> KPEPTDEEWELIKTVTEAHVATNAQGSHWKQKRKFLPEDIGQAPIVNAPEGGKVDLEAFSHFTKIITPAITRVVDFAKKLPMFCELPCEDQIILLKGCCMEIMSLRAAVRYDPESETLTLNGEMAVTRGQLKNGGLGVVSDAIFDLGMSLSSFNLDDTEVALLQAVLLMSSDRPGLACVERIEKYQDSFLLAFEHYINYRKHHVTHFWPKLLMKVTDLRMIGACLASRFLHMKVECPTELFPPLFLEVF;> ENALLRYLLDK

The thyroid hormone receptors (THRs) are nuclear hormone receptors regulated by endogenous thyroid hormones, including the inactive prohormone thyroxine (T4) and the bioactive hormone 3,3′,5-triiodothyronine (T3), which are critical for development regulation and metabolic homeostasis. As ligand-regulated nuclear receptors, THRs have a structurally conserved LBD that allows the binding of distinct ligands (Burris et al., 2013). Following the ligand binding, the function of THRs is mediated through the selective recruitment or release of specific coregulators, like the family of steroid receptor coactivators (SRCs) (Li et al., 2003, Jin and Li, 2010, Savkur and Burris, 2004), as a heterodimeric complex with retinoid X receptor (RXR) (Putcha et al., 2012, Kojetin et al., 2015, Mangelsdorf and Evans, 1995). Although the defects in any of the processes in thyroid hormone transport and synthesis can all contribute to RTH, in most cases the disorder involves defective thyroid hormone receptors, resulting in reduced T3 binding and disruptive thyroid hormone signaling.

As expected, the native ligand T3 abolished or substantially diminished the transcriptional activity of four THRβ mutants associated with thyroid hormone resistance, V264D, H435L, R438H, and R438W, respectively (Wakasaki et al., 2016, Nomura et al., 1996, Sabet and Pallotta, 2011, Narumi et al., 2010). Surprisingly, the treatment of roxadustat either enhanced or retained the transcriptional activity of these THRβ mutants, all leading to higher induced transcriptional activity than those of T3. In contrast, the binding of roxadustat resulted in higher Tm values for four TRβ mutants than that of T3. Although all four mutant residues are located in the THRβ LBD, H435 is the only one that directly contacts ligands T3 or roxadustat, whereas the rest of the mutant residues are located outside the ligand-binding pocket, not in the range to form intimate contacts with the ligands, which makes us wonder how these mutants influence the ligand binding. To unravel the molecular basis for the RTH of the THRβ mutants and further their beneficial susceptibility to roxadustat, we performed structural studies on the THRβ mutants complexed with roxadustat. The structural analysis further revealed an apparent conformational change of residue H435 on helix 10 of THRβ for all four mutants, resulting in the loss of a critical hydrogen bond between THRβ and a critical hydroxy group of T3, which is also conserved for the other THR ligands identified so far, explaining the severely reduced THRβ activity by T3. Specifically, in addition to the direct mutation of H435 to the hydrophobic leucine of THRβ H435L, the allosteric conformational changes of THRβ H435 were coupled with several intermediate structural changes, predominantly in helix 10, which were initiated by mutants R438H, R438W, or V264D, consequently leading to impaired T3 binding.> GMTYELSTDREFDLIAIGRACIDLNAVEYNRPMEETMTFSKYVGGSPANIVI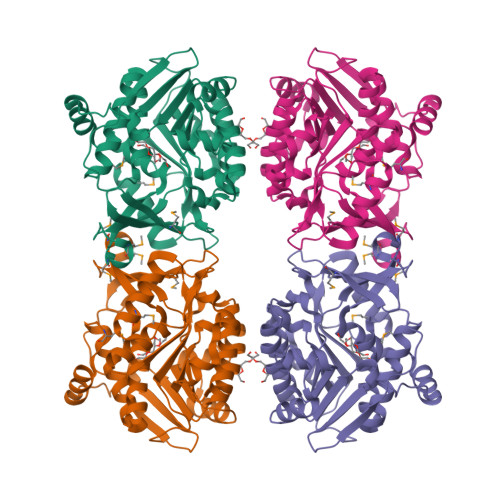GSSKLGLKAGFIGKIADDQHGRFIESYMRGVGVDTSNLVVDQEGHKTGLAFTEIKSPEECSILMYRQDVADLYLSPEEVNEAYIRRSKLLLVSGTALSKSPSREAVLKAIRLAKRNDVKVVFELDYRPYSWETPEETAVYYSLVAEQSDIVIGTREEFDVLENRTEKGDNDETIRYLFKHSPELIVIKHGVEGSFAYTKAGEAYRGYAYKTKVLKTFGAGDSYASAFLYALISGKGIETALKYGSASASIVVSKHSSSDAMPSVEEIEALIEKDETITIA>HHHHHHMATETNYPVPYRSKLTEPFEPGQTLIIKGKTAEDSVRFTINLHNTSADFSGNDVPLHISVRFDEGKIVFNTFSKGEWGKEERKSNPYKKGDDIDIRIRAHDSKFSISVDQKEVKEYEHRVPLSSVTHFSVDGDILITYIHWGGKYYPVPYESGLAGDGLAPGKSLLIFATPEK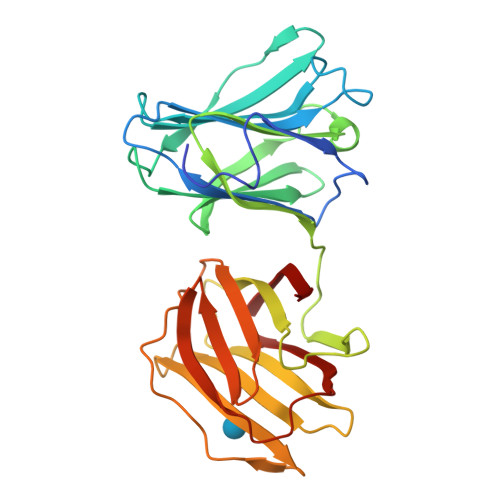KGKRFHINLLKKNGDIALHFNPRFDEKAIVRNSLISGEWGNEEREGKNPLEKGIGCDLEFRNEEYAFQIYVDGERFATYAHRLDPHDINGLQIGGDVEVTGIQMV[4x]>MLEYISSLPKQPISEEEKEGLIEMREEEKLARDVYLTLYNKWKLQIFKNIAESEQTHMDAVKYLLEKYNIPDPVKNDSIGVFSNPKFEELYKKLVEKGDKSEVDALKVGATIEDLDIADLEKWINKTDNEDIKFVYENLMKGSRNHMRAFVRMLNNYGSNYTPQYISKEEYEEIISSSTERGM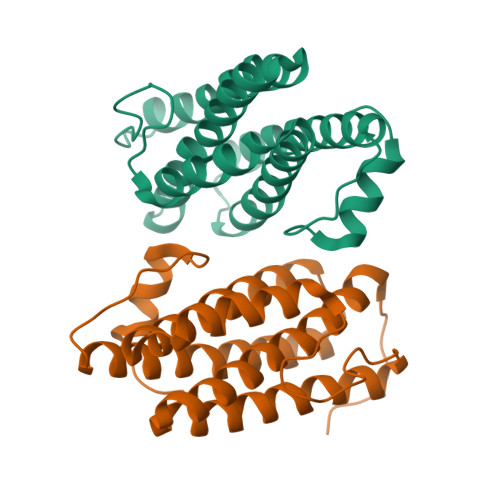NRLEHHHHHH[2x]> SVRKFTEKHEWVTTENGVGTVGISNFAQEALGDVVYCSLPEVGTKLNKQEEFGALESVKAASELYSPLSGEVTEINKALAENPGLVNKSCYEDGWLIKMTFSNPSELDELMSEEAYEKYIKSIEE

The bovine H-protein is a monomeric protein of molecular weight ∼14 kDa that plays a central role in the glycine cleavage system. The lipoic acid prosthetic group, covalently bound to Lys59 of the H-protein, interacts with specific sites on the P-, T- and L-proteins. The gene for bovine H-protein was isolated from a bovine liver cDNA library, and the purified recombinant apo H-protein can be lipoylated and activated in vitro by lipoyltransferase, using lipoyl-AMP as the lipoyl donor.

In this study, we applied the high-pressure cryocooling method to crystals of bovine H-protein, and determined the X-ray crystal structure at 0.86 Å resolution. The high-pressure cryocooled crystal of bovine H-protein belonged to space group C2 with unit-cell dimensions of a = 84.73, b = 41.40, c = 43.28 Å, β = 91.57°. The differences in unit-cell dimensions were less than 0.5%, even though the crystals of bovine H-protein had a high solvent content of ∼55%. The interactions and the positions of water molecules for crystal packing were perfectly conserved between high- and ambient-pressure crystals. The final model consists of 1172 protein atoms, 300 water molecules and two glycerol molecules. Hydrogen atoms were observed as peaks in a hydrogen-omit electron density map calculated at 0.86 Å resolution, and 48.9% of the hydrogen atoms could be visualized. Multiple conformations were observed for 31 residues, and 23 residues shared multiple conformations with the ambient-pressure structure. The r.m.s. deviation for Cα atoms is 0.12 Å, and the r.m.s. deviation for all atoms was 0.61 Å. In the high-pressure cryocooling structure, 196 of 300 water molecules were in common with water molecules in the ambient-pressure structure, and the r.m.s. deviation was 0.48 Å. We observed no significant differences in structural comparisons at ultra-high resolution, and there seemed to be no artificial structural variation resulting from the high-pressure cryocooling.>MTKQAEETQKPIIFAPETYQYDKFTLNEKQLTDDPIDLFTKWFNEAKEDPRETLPEAITFSSAELPSGRVSSRILLFKELDHRGFTIYSNWGTSRKAHDIATNPNAAIVFFWKDLQRQVRVEGITEHVNRETSERYFKTRPRGSKIGAWAS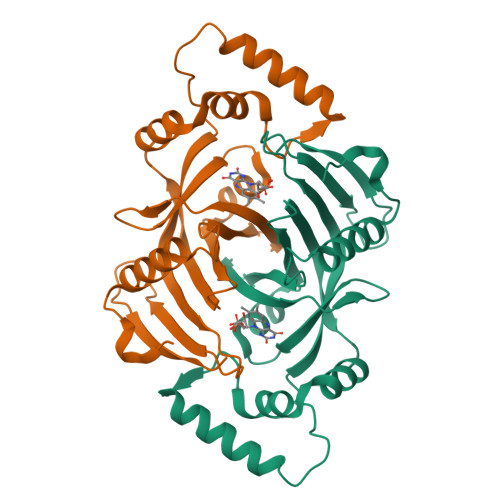RQSDVIKNREELDELTQKNTERFKDAEDIPCPDYWGGLRIVPLEIEFWQGRPSRLHDRFVYRRKTENDPWKVVRLAP[2x]>[2x]MTTVRIPAGWPATEEEARAVQDELRGRVILDEPGPPPGTGRVTGVDVAYDDERDVVVAAAVVLDAATLDVVAEATAVGEVSFPYVPGLLAFREIPTVLA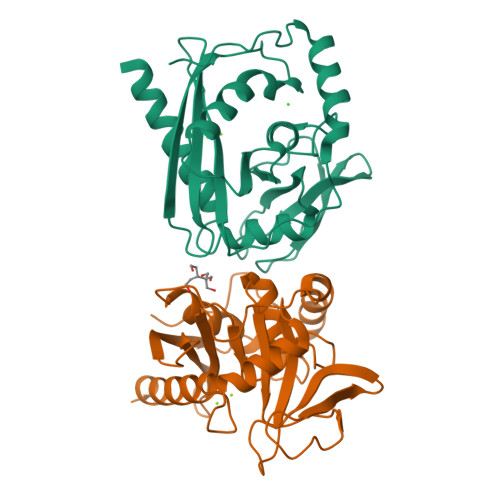ALDALPCPPGLIVCDGYGVAHPRRFGLASHLGVLTGLPTIGVAKNPFTFSYEDPGAPRGSAAPLLAGADEVGRALRTQSGVKPVFVSVGHRVDLDHACAHTLALTPKYRIPETTRRADSLCRRALKEATALEHHHHHH> ARMLAERQAKVRALVEAAHGLVEHQGARAARGEISADEARRAALEALRALRYDGSEYFWVNDLEPRMVMHPTNPQLDGQ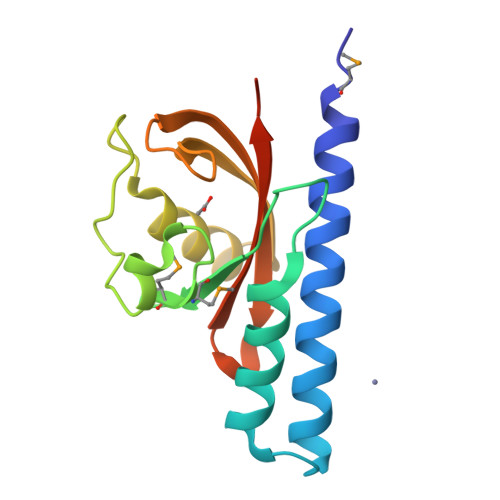DLSGYRDPNGKLLFQEFVRTVRARGSGFVDYLWPKPGSTVPVPKISFVTQYQPWGWVVGSGLYVDDLDAAVRQE>PTPCYISIEGQTQGLITAGACTADSIGDSFVEGHEDEMLVQQFDHVVTVPTDPQSGQPSGQRVHKPFKFTVALNKAVPLLYNALSSGEKLKTVELKWYRTSIEGKQENFFTTKLENASIVDIHCEMPHCQDPAKSDFTQNVTVSLSYRKITWDHVNAGTSGSDDWRKPIE[6x];>GSLLDEIMAQTRIAPSEEGYDIAKKGVAAFIENLMGSQHSAEPVNKSLVDQMLVELDKKISAQMDEILHNSQFQAMESAWRGLKLFVDRTDFRENNKVEILHVTKDELLEDFEFAPETAQSGLYKHVYSAGYGQFGGEPVGAIIGNYAFTPSTPDMKLLQYMGALGAMAHAPFISSVGPEFFGIDSFEELPNIKDLKSTFESPKYTKWRSLRESEDARYLGLTAPRFLLRVPYDPIENPVKSFNYAENVSASHEHYLWGNTAFAFATRLTDSFAKYRWCPNIIGPQSGGAVEDLPVHVFESMGALQSKIPTEVLITDRKEFELAEEGFIALTMRKGSDNAAFFSANSIQKPKVFPNTKEGKEAETNYKLGTQLPYMMIINRLAHYVKVLQREQIGAWKERQDLERELNSWIKQYVADQENPPADVRSRRPLRAARIEVMDVEGNPGWYQVSLSVRPHFKYMGANFELSLVGRL[6x];>SKEGSVAPKERIN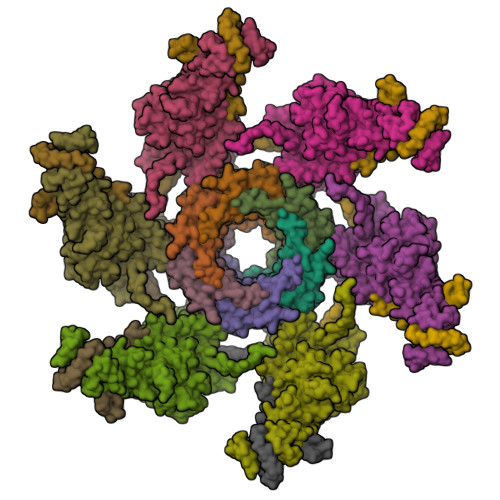IKYIPATGDAQAEVAEVELPLKTLVVGDFKGHAEQTPLEERATVTVDKNNFEAVMRESELKITATVKNKLTDDENAELPVELNFKSLADFAPDAVASQVPELKKLIELREALVALKGPLGNIPAFRERLQSLLNSEESREKLLAEL[6x]>MELWLVRHGETLWNREGRLLGWTDMPLTAEGEAQARRLKGALPSLPAFSSDLLRARRTAELAGFSPRLYPELREIHFGALEGALWETLDPRYKEALLRFQGFHPPGGESLSAFQERVFRFLEGLKAPAVLFTHGGVVRAVLRALGEDGLVPPGSAVAVDWPRRVLVRLALDGEEAT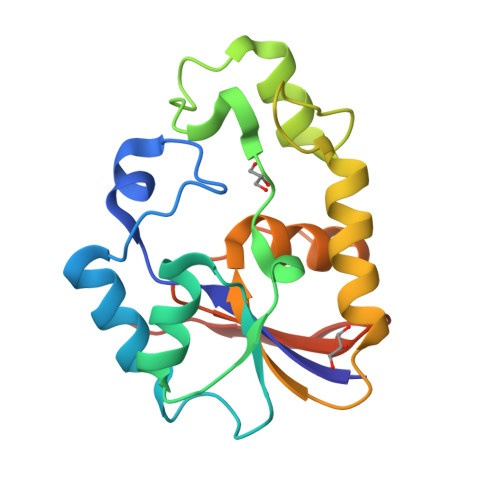G[2x]>MIPGKPWDTPQLAAELERWKLDGRDVSLLIGGPEGLSPACKAAAEQSWSLSALTLPHPLVRVLVAESLYRAFSITTNHPYHREGSMKLQLVAVGTKMPDWVQTGFTEYLRRFPKDMPFELIEIPAGKRGKNADIKRILDKEGEQMLAAAGKN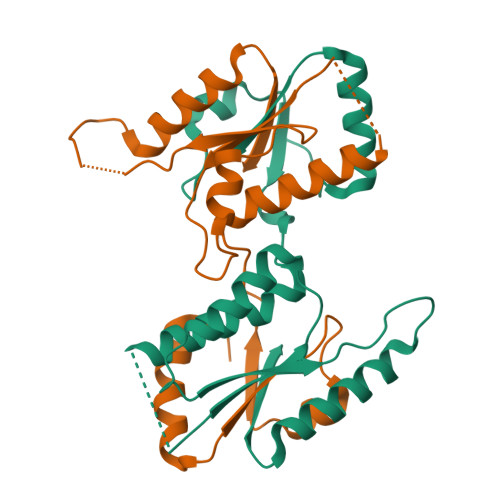RIVTLD[2x]> GKMKKDYRKKYRKYVRSRFQCIEDRNARLGESVSLNKRYTRLRLIKEHRSQQEREQELLAIGKTKTCESPVSPIKMELLFDPDDEHSEPVHTVVFQGAAGIGKTILARKMMLDWASGTLYQDRFDYLFYIHCREVSLVTQRSLGDLIMSCCPDPNPPIHKIVRKPSRILFLMDGFDELQGAFDEHIGPLCTDWQKAERGDILLSSLIRKKLLPEASLLITTRPVALEKLQHLLDHPRHVEILGFSEAKRKEYFFKYFSDEAQARAAFSLIQENEVLFTMCFIPLVCWIVCTGLKQQMESGKSLAQTSKTTTAVYVFFLSSLLQPRGGSQEHGLCAHLWGLCSLAADGIWNQKILFEESDLRNHGLQKADVSAFLRMNLFQKEVDCEKFYSFIHMTFQEFFAAMYYLLEEEKEGRTNVPGSRLKLPSRDVTVLLENYGKFEKGYLIFVVRFLFGLVNQERTSYLEKKLSCKISQQIRLELLKWIEVKAKAKKLQIQPSQLELFYCLYEMQEEDFVQRAMDYFPKIEINLSTR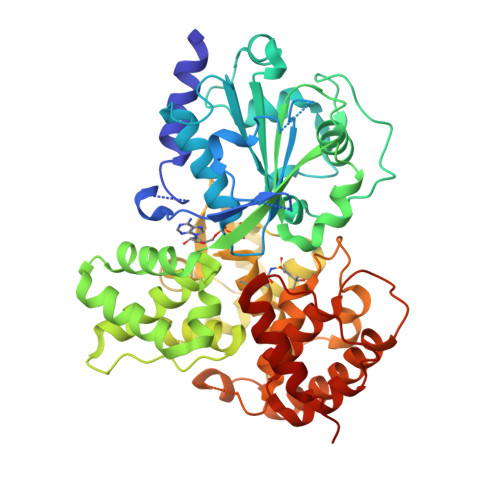MDHMVSSFCIENCHRVESL>ADEIAKAQVARPGGDTIFGKIIRKEIPAKIIFEDDRCLAFH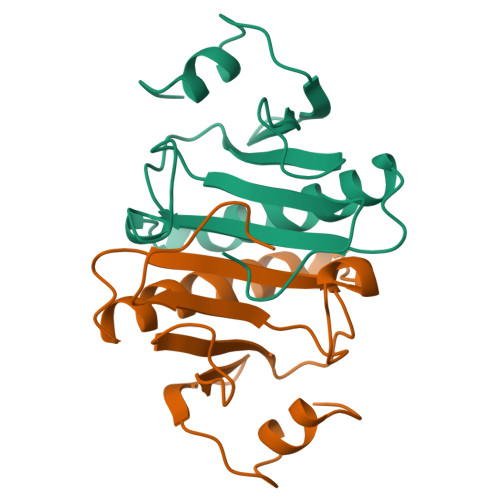DISPQAPTHFLVIPKKHISQISVAEDDDESLLGHLMIVGKKCAADLGLNKGYRMVVNEGSDGGQSVYHVHLHVLGGRQMHWPPG[2x]[2-(3,5-DI-TERT-BUTYL-4-HYDROXY-PHENYL)-1-(DIETHOXY-PHOSPHORYL)-VINYL]-PHOSPHONIC ACID DIETHLYL ESTER | C24 H42 O7 P2 | 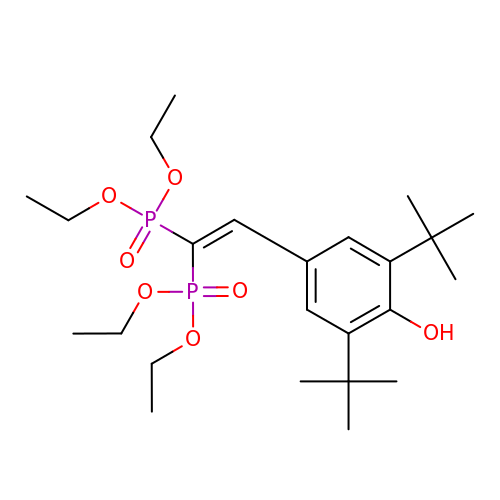YQLJDECYQDRSBI-UHFFFAOYSA-N> MKTLIIETANAKILGELVTVSRLFGQAPDVVVLGSGELQGSYGKAYRLSDTLGANLGSSLSDLIKRERYELILLSTTAIGSGLAGPLAVSLGAPILSEVTAISPDLTIERSLYGSKAVARYKLESGPLVLTIKRKYFEAATLEGTTATEELPVGPQKITLLEEIEEERTGIPLEDAEVVVTGGRGIGSGDNFSILKEIAGMLNGAVGASRGAVDEGWMPPGAQIGQTGKIVAPTVYFAVGVSGASQHLAGISNAKCVIAINKDNEANIFKRARFGIVGDYKKAVPALINALKEN;> MQIVVLAKVVPDYEVPSADFELVGNRAHPRYTRMIGLYDENAVELGVQLKEKLGADLTVVSYGRNDDVQFLRKALAMGADKVVLVEGDSDDPYVIAANLKDAIDRQGTVDLILAGRQSSDMDRGVVPGVLAGMLDLPFVPQACSVESVDGGWKISQITETGKRLLKLSGKGVLSITSVPENVPRIPAVKAIFAAKKKPVE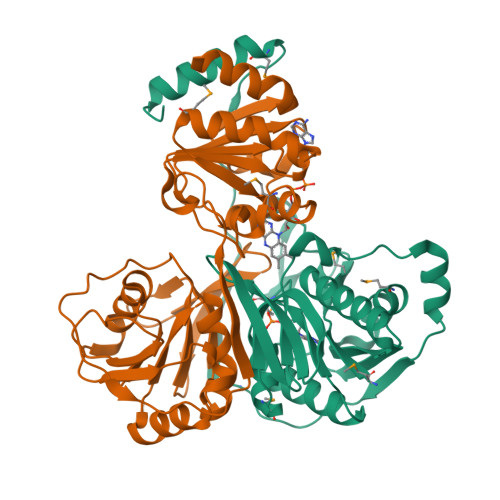KLPEIGTGKMAVSELSVSIPKVESNCELIPAEDMDDAVRVLLRRLKEERYL>MSKLVLTGERHYTRNDDIRQSILALGEPGTFMTQDVNIIQTQIEQRLPWIKQVSVRKQWPDELKIHLVEYVPIARWNDQHMVDAEGNTFSVPPERTSKQVLPMLYGPEGSANEVLQGYREMGQMLAKDRFTLKEAAMTARRSWQLTLNNDIKLNLGRGDTMKRLARFVELYPVLQQQAQTDGKRISY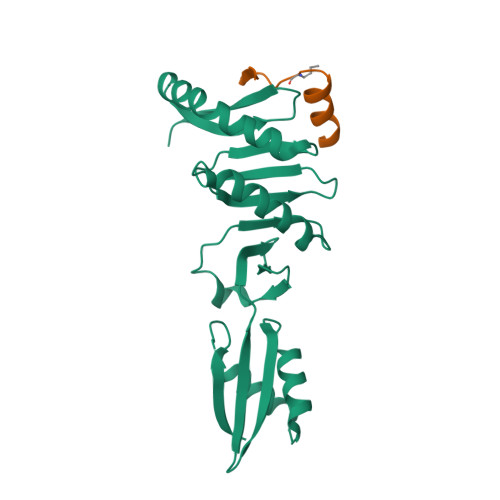VDLRYDSGAAVGWAPLPPEESTQQQNQAQAEQQGSHHHHHH[2x];>QEALEERARNELSLTRPGETFYRL[2x]>MPLSAFSPPLPCDPARSHPTPEFPSSLQDYCEIRGIQSQPPARRDPTMDWLASLRSQIKPYRDRFPSHARLPRAGLPRAEILAEIAAMGAAESPAWRDGYASGAVYHGDEHHIAFLNEVYALQSQSNPLHPDLWPSTAKFEAEVVAMTAHMLGGDAAGGTVCGTVTSGGTESLLLAMKTYRDWARATKGITAPEAVVPVSAHAAFDKAAQYFGIKLVRTPLDADYRADVAAMREAITPNTVVVAGSAPGFPHGVVDPIPEIAALAAEHGIGCHVDACLGGFILPWAERLGYPVPPFDFRLEGVTSVSADTHKYGYGAKGTSVILYRRPDLLHYQYFIAADWPGGIY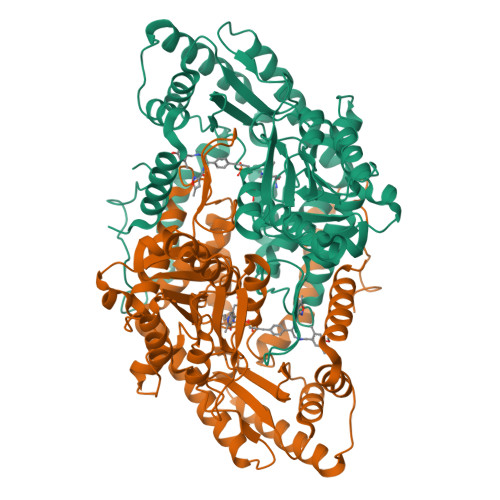ASPTFAGSRPGALSATAWAAMLSLGEEGYLDATRRILQAADRLKAGVRAIPSLKILGDPLWVIAVASDELNIYQVMEEMAGRGWRLNGLHRPPAFHVALTLRHTEPGVVDRFLADLQDAVAQVRAHPEKATGMAPVYGMAAAAPPELVRQVSTGFIDLLYEVHHHHHH[2x]> YEASILTHDSSIRYLQEIYNSNNQKIVNLKEKVAQLEAQCQEPCKDTVQIHDITGKDCQDIANKGAKQSGLYFIKPLKANQQFLVYCEIDGSGNGWTVFQKRLDGSVDFKKNWIQYKEGFGHLSPTGTTEFWLGNEKIHLISTQSAIPYALRVELEDWNGRTSTADYAMFKVGPEADKYRLTYAYFAGGDAGDAFDGFDFGDAPSAKFFTSHNGMQFSTWDNDNDKFEGNCAEQDGSGWWMNKCHAGHLNGVYYQGGT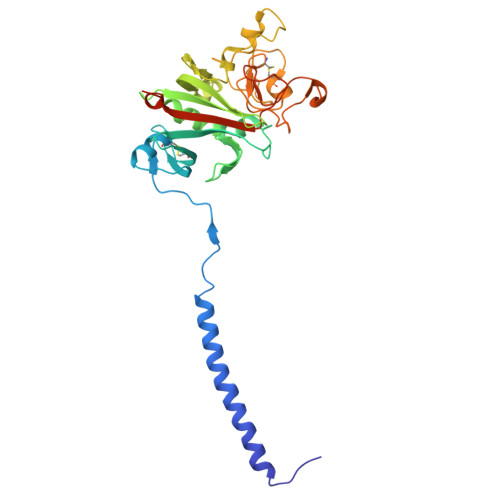YSKASTPNGYDNGIIWATWKTRWYSMKKTTMKIIPFNRLTIGEGQQHHLGGAK>ASASAFWLEVEGNSMTAPTGSKPSFPDGMLILVDPEQ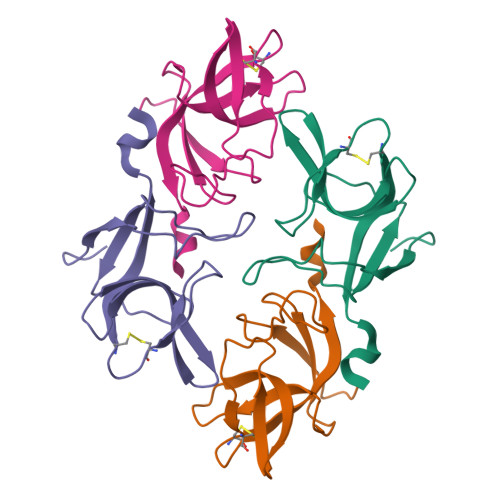AVEPGDFCIARLGGDEFTFKKLIRDSGQVFLQPLNPQYPMIPCNESCSVVGKVIASQWPEETFG[2x]> MNQTLETGTTTVGITLKDAVIMATERRVTMENFIMHKNGKKLFQIDTYTGMTIAGLVGDAQVLVRYMKAELELY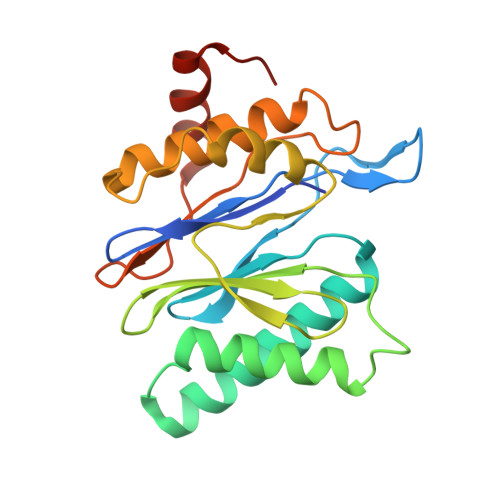RLQRRVNMPIEAVATLLSNMLNQVKYMPYMVQLLVGGIDTAPHVFSIDAAGGSVEDIYASTGSGSPFVYGVLESQYSEKMTVDEGVDLVIRAISAAKQRDSASGGMIDVAVITRKDGYVQLPTDQIESRIRKLGLILHHHHHH>[2x]ADAEHVVEARKGYFSLVALEFGPLAAMAKGEMPYDAAAAKAHASDLVTLTKYDPS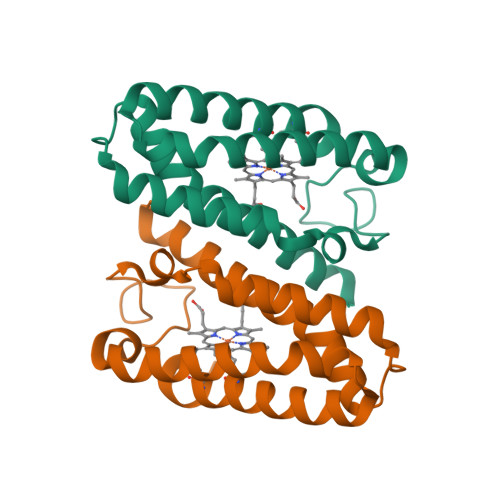DLYAPGTSADDVKGTAAKAAIWQDADGFQAKGMAFFEAVAALEPAAGAGQKELAAAVGKVGGTCKSCHDDFRVKR> MEDTETSLVASPTDQQVSLFRYITQAVVTAPRAKDPANP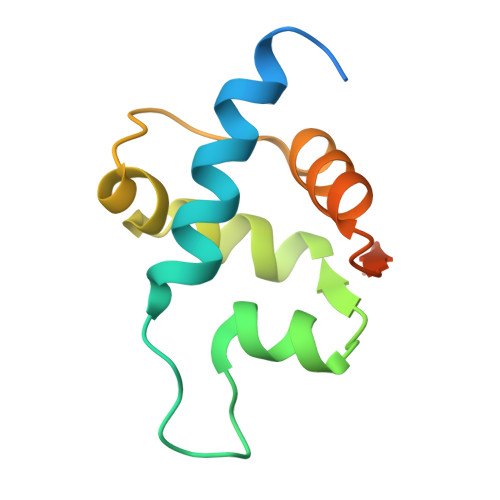SWHEKMLMYDPIILEDLTAWLNSGQLDRVGYDGEVAPGDVKKWCESKSVCCLWRVSLNGKERKRF> GHEIKDIREDTMHAEFNALRAQVAINDGNPDEAERLAKLALEELPP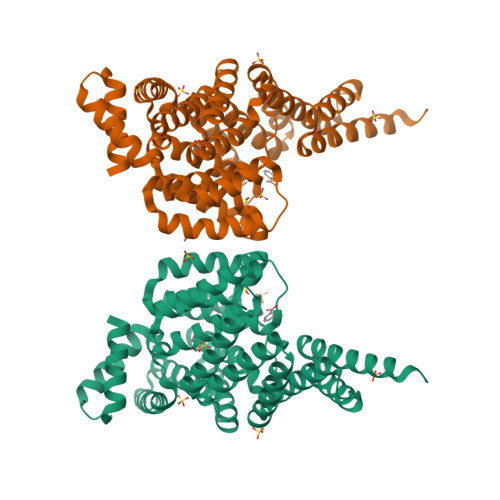GWFYSRIVATSVLGEVLHCKGELTRSLALMQQTEQMARQHDVWHYALWSLIQQSEILFAQGFLQTAWETQEKAFQLINEQHLEQLPMHEFLVRIRAQLLWAWARLDEAEASARSGIEVLSSYQPQQQLQCLAMLIQCSLARGDLDNARSQLNRLENLLGNGKYHSDWISNANKVRVIYWQMTGDKAAAANWLRHTAKPEFANNHFLQGQWRNIARAQILLGEFEPAEIVLEELNENARSLRLMSDLNRNLLLLNQLYWQAGRKSDAQRVLLDALKLANRTGFISHFVIEGEAMAQQLRQLIQLNTLPELEQHRAQRILREINQHHGA>MQIQTDVVLPSCKKKAPAETPVKERLFIVFNPHPLPLDVLEDIFCRFGNLIEVYLVSGKNVGYAKYA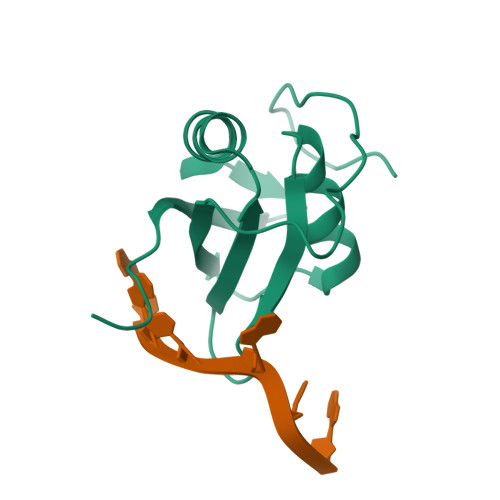DRISANDAIATLHGKILNGVRLKVMLADSPREESNKRQRTYLEHHHHHH[4x]> ISEFDYKDHEIDYKDDDDKWIMSLSIKELYYTKDKSINNVNLADGNYVVNRGDGWILSRQNQNLGGNISNNGCTAIVGDLRIRETATPYYYPTASFNEEYIKNNVQNVFANFTEASEIPIGFEFSKTAPSNKSLYMYLQYTYIRYEIIKVLQNTVTERAVLYVPSLGYVKSIEFNSEEQIDKNFYFTSQDKCILNEKFIYKKIDD;> QTILPYPNGLYVINKGDGYMRTNDKDLIGTL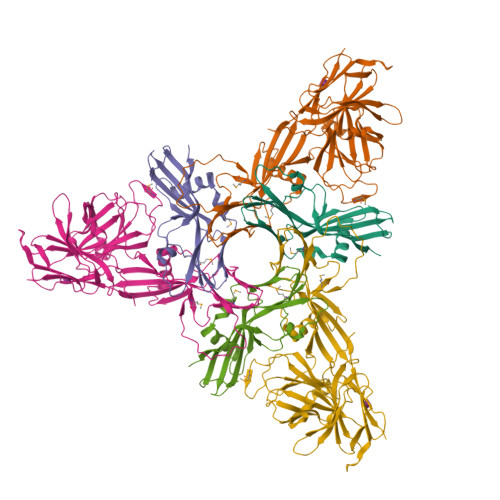LIESSTSGSIIQPRLRNTTRPLFNTSNPTIFSQEYTEARLNDAFNIQLFNTSTTLFKFVEEAPTNKNISMKVYNTYEKYELINYQNGNIDDKAEYYLPSLGKCEVSDAPSPQAPVVETPVDQDGFIQTGPNENIIVGVINPSENIEEISTPIPDDYTYNIPTSIQNNACYVLFKVNTTGVYKITTKNNLPPLIIYEAIGSSNRNMNSNNLSNDNIKAIKYITGLNRSDAKSYLIVSLFKDKNYYIRIPQISSSTTSQLIFKRELGNISDLADSTVNILDNLNTSGTHYYTRQSPDVGNYISYQLTIPGDFNNIASSIFSFRTRNNQGIGTLYRLTESINGYNLITINNYSDLLNNVEPISLLNGATYIFRVKVTELNNYNIIFDAYRNS> MKLKLIVNGCEAPDDYKLLRTTINTVASLRKTAILRFNSERLTIISTPKSSLNSSNNGTILRGDTGQLWCTIPHDVFRLYTVISARELNTITMECNCDSLLSVFKRYDRVMNQGSSSNMTIKLQSMPEWNTNNGTLSGGTAGGVDTTSKPNPICALGITFEEIVHTSGPNDAIVMNGGVDEHNGLPTTVGTGNL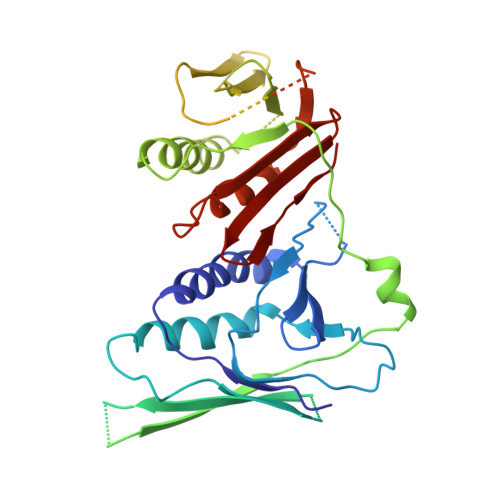LASNKVIMHSFKVPVKLLFRAQDTRIQEPMINYIQLMMYKLPPISGEFGSAFHGFIRRVERYSNVNHIHLMGVKKKEHGNEGDDVELKIIVNELDWHLEICWNGPLDSVIQRQEGLTDNPSQNQHIDTDGRQEEGSLPIIEADKPMSSLYTNTRDREMEENIRYDEDLLRIEDSSIADTRGNIYTADTSGDTEFNDISVMVEKAEQESSSTHEVIIRCKDWKVCSKLYAAFEEVVLAISHDESCVFHCSLDERGQIIYYIARSKGL>[4x]MKCLKAVIPVAGLGTRMLPATKAIPKEMLPVVDKPLIQYIVDECVAAGVKEIVLVSHSSKNAIENHFDTSFELEAALESRVKRQLLKEIKNICPADVTIMQVRQGHAKGLGHAVLCAKSMVGDNPFI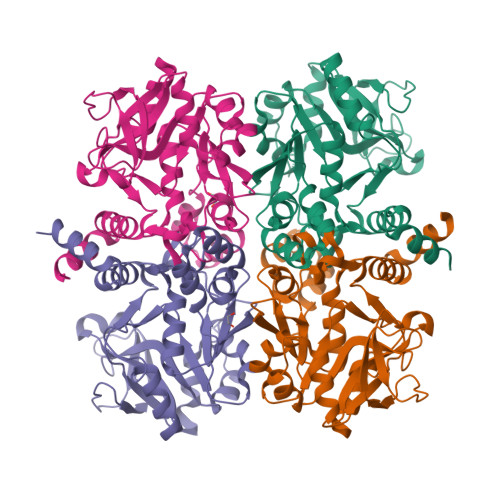VMLPDVLLDDSTADLSKENLASMIKRFEETGHSQIMVEPVPKADVSKYGIADCGHVALAPGESTLMTAVVEKPSIAEAPSNLAVVGRYVLSKNIWPLLEKTPRGAGDEIQLTDAIAMLMQQEPVEAFHMTGKSHDCGDKLGYMKAFVTYGVRHHTEGEKFTAWLKQQLD>[2x]MLQKLIQILRRNEYVKNVYKNTVSNFIETSIPEITPFNARTSSIKGKRLNLLVP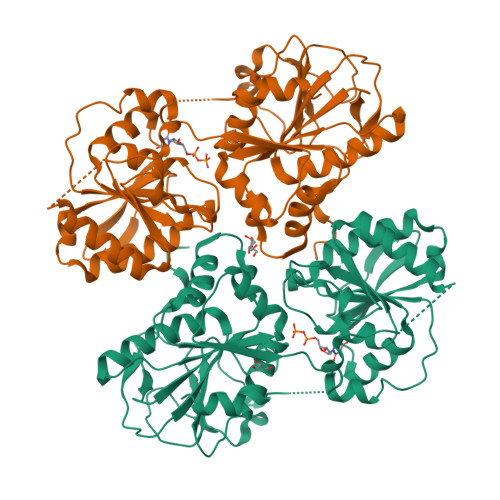SINQEHMFGGISTALKLFEQFDNAAFAKRIILTDATPNPKDLQSFKSFKYVMPEEDKDFALQIVPFNDRYNRTIPVAKHDIFIATAWWTAYAAQRIVSWQSDTYGIPPNKILYIIQDFEPGFYQWSSQYVLAESTYKYRGPQIAVFNSELLKQYFNNKGYNFTDEYFFQPKINTTLKNYINDKRQKEKIILVYGRPSVKRNAFTLIVEALKIFVQKYDRSNEWKIISVGEKHKDIALGKGIHLNSLGKLTLEDYADLLKRSSIGISLMISPHPSYPPLEMAHFGLRVITNKYENKDLSNWHSNIVSLEQLNPENIAETLVELCMSFNNRDVDKKESSNMMFYINEFNEFSFIKEIEEKL> GSMIDKSAFVHPTAIVEEGASIGANAHIGPFCIVGPHVEIGEGTVLKSHVVVNGHTKIGRDNEIYQFASIGEVNQDLKYAGEPTRVEIGDRN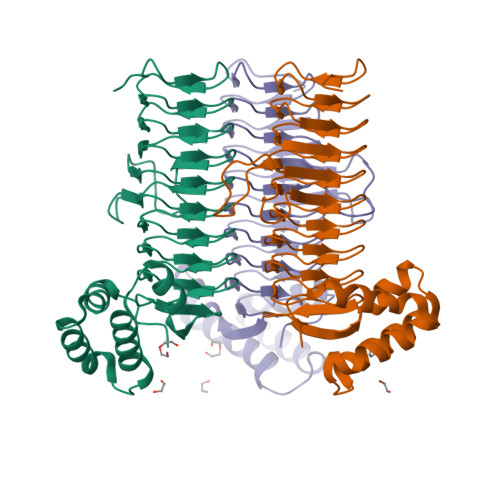RIRESVTIHRGTVQGGGLTKVGSDNLLMINAHIAHDCTVGNRCILANNATLAGHVSVDDFAIIGGMTAVHQFCIIGAHVMVGGCSGVAQDVPPYVIAQGNHATPFGVNIEGLKRRGFSREAITAIRNAYKLIYRSGKTLDEVKPEIAELAETYPEVKAFTDFFARSTRGLIR> AEIYNKDGNKVDLYGKAKGLHYFSKGNGENSYGGNGDMTYARLGFKGETQINSDLTGYGQWE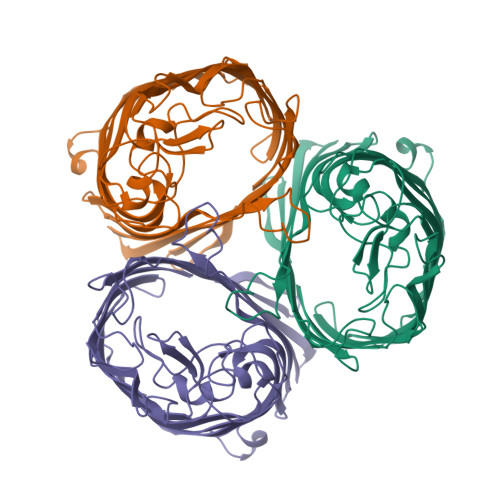YNFQGNNSEGADAQTGNKTRLAFAGLKYADVGSFDYGRNYGVVYDALGYTDMLPEFGGDTAYSDDFFVKRVGGVATYRNSNFFGLVDGLNFAVQYLGKNERDTARRSNGDGVGGSISYEYEGFGIVGAYGAADRTNLQEAQPLGNGKKAEQWATGLKYDANNIYLAANYGETRNATPITNKFTNTSGFANKTQDVLLVAQYQFDFGLRPSIAYTKSKAKDVEGIGDVDLVNYFEVGATYYFNKNMSTYVDYIINQIDSDNKLGVGSDDTVAVGIVYQF> XAEIAAIKYKQAAIKNEIAAIKQEI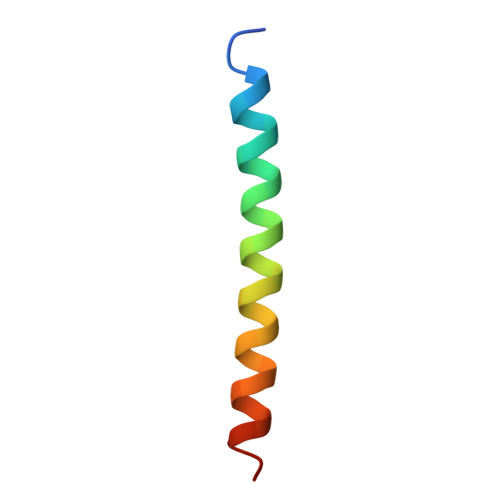AAIEQMIAAIX> MHHH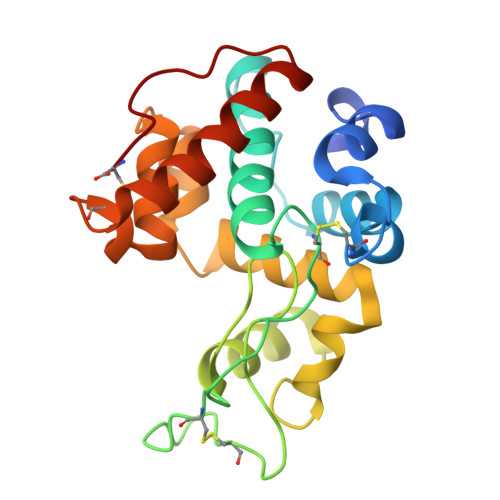HHHGVGSIVSSDVFNSIVGGAASGCAGNGFYTYDSFISAANAFNGFGTSGSSDVNKREIAAFFANAAHETGGFCYIEEQNPTSIYCDASNTQYPCASGKTYHGRGPLQLSWNYNYGAAGSYIQFDGLNNPEIVGTDSTISFKTAVWFWMVNSNCHTAITSGQGFGATIRAINSMECDGGNAATVASRVNYYQKFCQQLNVDTGSNLQC2-(1-DIMETHYLAMINOMETHYL-2-HYDROXY-8-HYDROXYMETHYL-9-OXO-9,11-DIHYDRO-INDOLIZINO[1,2-B]QUINOLIN-7-YL)-2-HYDROXY-BUTYRIC 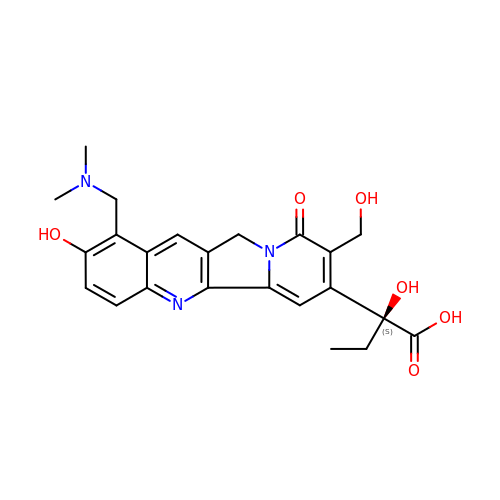ACID | C23 H25 N3 O6 | DPQJTQJZJNYUEC-QHCPKHFHSA-N> MNINDNLSINSPVDNKNVVVVRARKTDTVFKAFKVAPNIWVAPERYYGESLSIDEEYKVDGGIYDSNFLSQDSEKDKFLQAIITLLKRINSTNAGEKLLSLISTAIPFPYGYIGGGYYAPNMITFGSAPKSNKKLNSLISSTIPFPYAGYRETNYLSSEDNKSFYASNIVIFGPGANIVENNTVFYKKEDAENGMGTMTEIWFQPFLTYKYDEFYIDPAIELIKCLIKSLYFLYGIKPSDDLVIPYRLRSELENIEYSQLNIVDLLVSGGIDPKFINTDPYWFTDNYFSNAKKVFEDHRNIYETQIEGNNAIGNDIKLRLKQKFRININDIWELNLNYFSKEFSIMMPDRFNNALKHFYRKQYYKIDYPENYSINGFVNGQINVQLSLSDRNQDIINKPEEIINLLNGNNVSLMRSNIYGDGLKSTVDDFYSNYKIPYNRAYEYHFNNSNDSSLDNVNIGVIDNIPEIIDVNPYKENCDKFSPVQKITSTREINTNIPWPINYLQAQNTNNEKFSLSSDFVEVVSSKDKSLVYSFLSNVMFYLDSIKDNSPIDTDKKYYLWLREIFRNYSFDITATQEINTDCGINKVVTWFGKALNILNTSDSFVEEFQNLGPISLINKKENLSMPIIEIYGIPNDMLGLPLNDLNEKLFNIYLKNILYFKKVYFNFLDQWWTEYYSQYFDLICMAKQSILAQEKLIKQIIQNKLQDLFKADISMDKLNLMNLATEKTFIDLSNESQIAINNINDFLNKSAICVFDTNIYPKFISFMEQCINSVNSNVTAFIQKCTNITEDEKLQLIKLNTFMNIDFEFFDIQSIKDLITSETDLIKEEKESDYNLFLFTLQEDNNKVIEDISGKNTLVKYSDSISLVYGVNGDALYLKEPDESVSFSNKAFENGLTNSFSICFWLRNLGEDIITSKLIENKADNCGWEIYFENNGLVFSIVDCNGNEENIYLSDVISKNWYYISISIDRLRNQLLIFINDKLIANQSIEQILNIYSSNTISLVNENNPIYIEGLSILNRSITSEEVVNNYFSYLNNSYIRDISGERLEYNKTYELYNYVFPENSLYEVTENNNIYLSI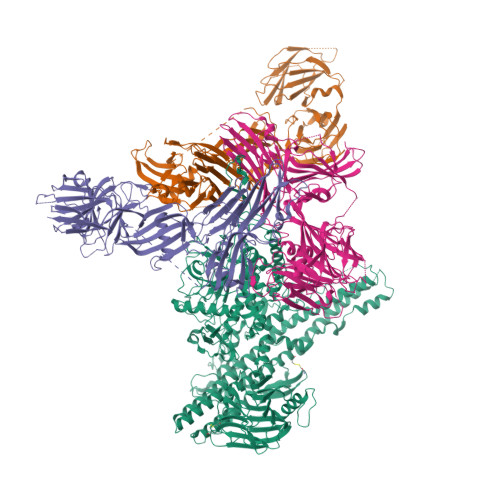KDTNNLNIQGAKFKLINIDANKQYVQKWDEGVVCLLGDEEKYVDISSENNRIQLVNSKDTAKRIIFNNDIFMPNCLTFAYNNKYLSLSLRDRNYNWMICNNNDNIPKAAHLWALKGI;>MNSSIKKIYNHIQEKVINYSDTIDLADGNYVVSRGDGWILSRQNQILGGSVISNGSTGIVGDLRVNDNAIPYYYPTPSFNEEYIKNNIQTVFANFTEANQIPIGFEFSKTAPSNKNLYMYLQYTYIRYEIIKVLQHEIIERAVLYVPSLGYVKSIEFNPGEKINKDFYFLTNDKCILNEQFLYKKILETTKNIPTNNIFNSKVSSTQRVLPYSNGLYVINKGDGYIRTNDKDLIGTLLIEAGSSGSIIQPRLRNTTRPLFTTSNDAKFSQQYTEERLKDAFNVQLFNTSTSLFKFVEEAPSNKNICIKAYNTYEKYELIDYQNGSIVNKAEYYLPSLGYCEVTNAPSPESEVVKTQVAEDGFIQNGPEEEIVVGVIDPSENIQEINTAISDNYTYNIPGIVNNNPFYILFTVNTTGIYKINAQNNLPSLKIYEAIGSGNRNFQSGNLCDDDIKAINYITGFDSPNAKSYLVVLLNKDKNYYIRVPQTSSNIENQIKFKREEGDLRNLMNSSVNIIDNLNSTGAHYYTRQSPDVHDYISYEFTIPGNFNNKDTSNIRLYTSYNQGIGTLFRVTETIDGYNLINIQQNLNLLNSTKSIRLLNGAIYILKVEVTELNNYNIKLHIDITN[3x]>MYKEPFGVKVDFETGIIEGAKKSVRRLSDMEGYFVDERAWKELVEKEDPVVYEVYAVEQEEKEGDLNFATTVLYPGKVGKEFFFTKGHFHAKLDRAEVYVALKGKGGMLLQTPEGDAKWISMEPGTVVYVPPYWAHRTVNIGDEPFIFLAIYPADAGHDYGTIAEKGFSKIVIEENG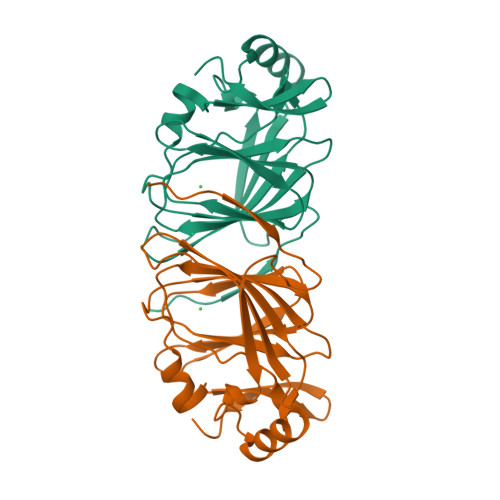EVKVVDNPRWKK[2x]(alpha-D-glucopyranosyloxy)acetic 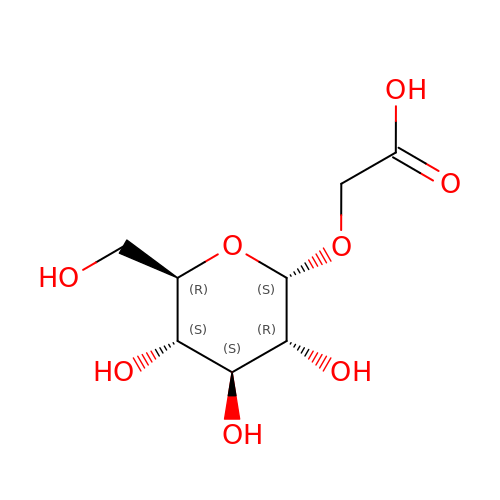acid | C8 H14 O8 | CEXKKLVRUODYGY-VDUCJHRSSA-N>MKHSHEEIRKIIPEMRRVQQIHFIGIGGAGMSGIAEILLNEGYQISGSDIADGVVTQRLAQAGAKIYIGHAEEHIEGASVVVVSSAIKDDNPELVTSKQKRIPVIQRAQMLAEIMRFRHGIAVAGTHGKTTTTAMISMIYTQAKLDPTFVNGGLVKSAGKNAHLGASRYLIAEADESDASFLHLQPMVSVVTNMEPDHMDTYEGDFEKMKATYVKFLHNLPFYGLAVMCADDPVLMELVPKVGRQVITYGFSEQADYRIEDYEQTGFQGHYTVICPNNERINVLLNVPGKHNALNATAALAVAKEEGIANEAILEALADFQGAGRRFDQLGEFIRPNGKVRLVDDYGHHPTEVGVTIKAAREGWGDKRIVMIF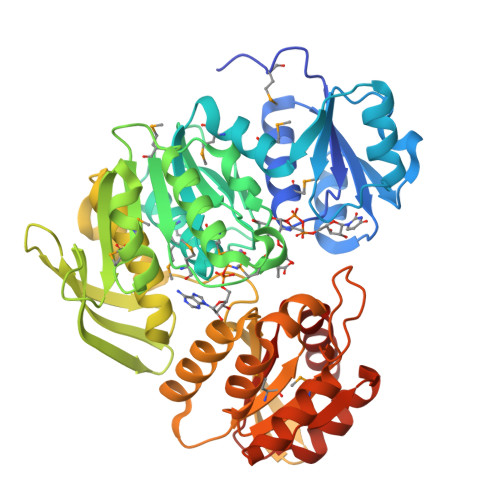QPHRYSRTRDLFDDFVQVLSQVDALIMLDVYAAGEAPIVGADSKSLCRSIRNLGKVDPILVSDTSQLGDVLDQIIQDGDLILAQGAGSVSKISRGLAESWKN[2x]> MAPTWFYNTTNSEKLRELQHVLGG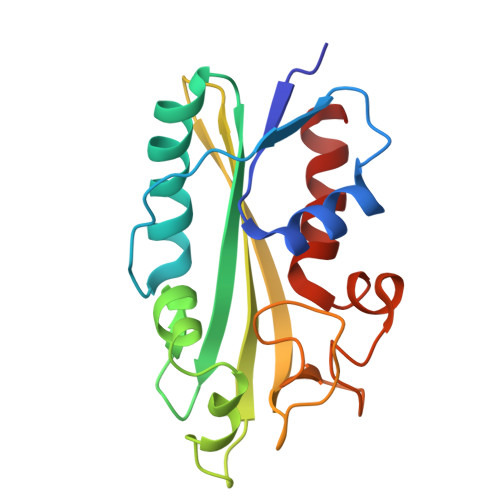SAKLGYLTAKVTEILDVDLETVIRAKAIAAYRAVRVPVIVEHGALCIDALNGLPGALVKPFWESLDTRLCEVIPAGQRTARARGALCYCDGRERHVLIEETEGEIAPSARGTGGFHWDPIFIPKGQTRTFAEMSLDEKLSFSPLGRLHTRLRTELGL> GSDFPSCRCVEQIIEKDEGPFYTHLGAGPNVAAIREIMEERFGQKGKAIRIERVIYTGKEGKSSQGCPIAKWVVRRSSSEEKLLCLVRERAGHTCEAAVIVILILVWEGIPLSLADKLYSELTETLRKYGTLTNRRCALNEERTCACQGLDPETCGASFSFGCSWSMYYNGCKFARSKIPRKFKLLGDDPKEEEKLESHLQNLSTLMAPTYKKLAPDAYNNQIEYEHRAPECRLGLKEGRPFSGVTACLDFCAHAHRDLHNMQNGSTLVCTLTREDNREFGGKPEDEQLHVLPLYKVSDVDEFGSVEAQE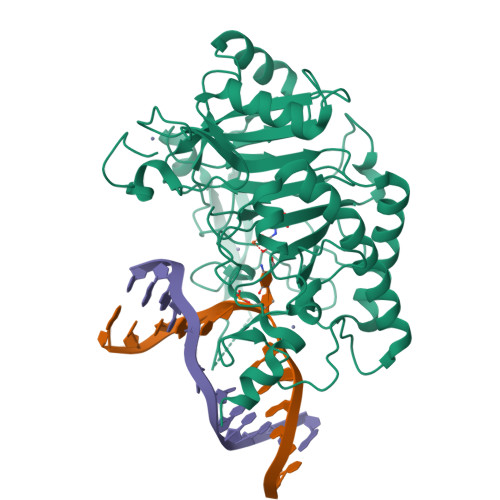EKKRSGAIQVLSSFRRKVRMLAEPVKTCRQRKLEAKKAAAEKLSGGGGSGGGGSGGGGSDEVWSDSEQSFLDPDIGGVAVAPTHGSILIECAKRELHATTPLKNPNRNHPTRISLVFYQHKSMNEPKHGLALWEAKMAEKAREKEEECEKYG>[3x]MNSKKSPVTLIGLGPMGQAMVRTLLGQGHPVTVWNRTPSRAEPLVVEGARLAASPTEAVASSDLVILSLTDYQAMYDILSTAESALAGRTIVNLSSDDPDVTREAAKWAAKHGATFIAG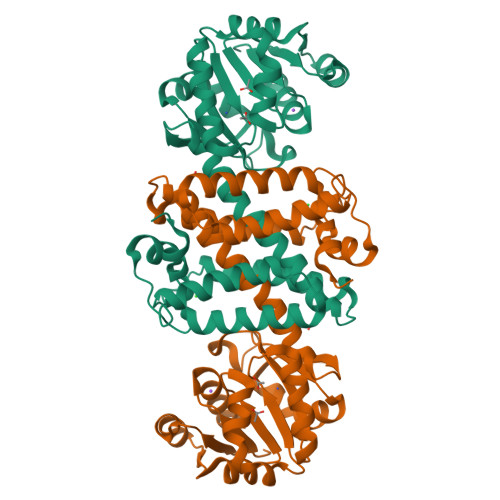GVMTPAPTVGTEAAYVFYSGPKSAFDAHEPVLRHIGGPRFLGEDTGLAQLYYLAHLDVFLTTLASVVHATALVSAAGVDEAAFAPEAIRMVIETGQMLAAEAETGLELGRNLASGNHPGELATAVMMGATADHIVSAAKGSGVDLVLPEAVKSLYDRTVAAGHGKDSWTAMYEIIKKKAA> MGSSHHHHHHSQDPNSMSQPFASRGLAWFQALAGSLAPRPGDPASLRVADAELDGYPVRFLAVVPDPDNPFPRARQGEVGLLEGWGLAAAVDEALEADREAPRKRALLAIVDVPSQAYGRREEALGIHQALAGAVDAYARARLAGHPLIGLLVGKAMSGAFLAHGYQANRLIALHDPGVMVHAMGKAAAARITLRSVEELEAL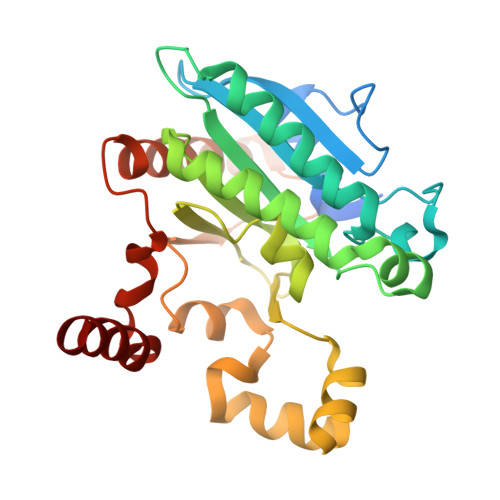AAKVPPMAYDIDSYASLGLLWRTLPVETVEVPSTADLVRVRTCLGEALADILGGPRDLGGRLGAANREASARVRRLLREQW>[4x]MDFVKELKSSQDYMNNELTYGAHNYDPIPVVLKRGKGVFVYDIEDRRYYDFLSAYSSVNQGHCHPDILNAMINQAKKLTICSRAFFSDSLGVCERYLTNLFGYDKVLMMNTGAEASETAYKLCRKWGYEVKKIPENSAKIIVCNNNFSGRTLGCVSASTD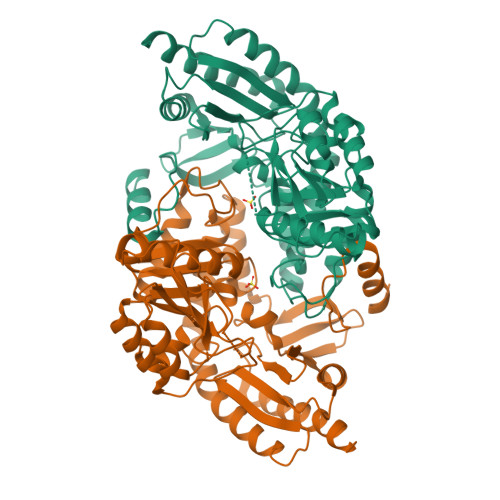KKCKNNFGPFVPNFLKVPYDDLEALEKELQDPNVCAFIVEPVQGEAGVIVPSDSYFPGVASLCKKYNVLFVADEVQTGLGRTGKLLCTHHYGVKPDVILLGKALSGGHYPISAILANDDVMLVLKPGEHGSTYGGNPLAAAICVEALKVLINEKLCENADKLGAPFLQNLKEQLKDSKVVREVRGKGLLCAIEFKNDLVNVWDICLKFKENGLITRSVHDKTVRLTPPLCITKEQLDECTEIIVKTVKFFDDNLLQHHHHHH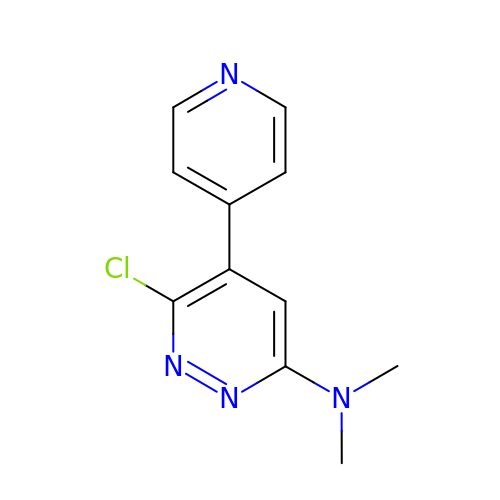6-chloro-N,N-dimethyl-5-(pyridin-4-yl)pyridazin-3-amine | C11 H11 Cl N4 | TXDDCILZWXYXEH-UHFFFAOYSA-N The set of protein arginine methyltransferases (PRMTs) is a family of enzymes that catalyze the transfer of a methyl group from S-adenosyl-L-methionine (SAM) to the guanidino nitrogen of an arginyl residue to produce S-adenosyl-L-homo-cysteine (SAH) and methyl arginyl residues. TbPRMT6 is the homologue of HsPRMT6 in T. brucei with 31% amino acid identity. The overall monomeric structure of TbPRMT6 consists of three parts: a SAM-binding domain (residues 36–181, blue), a dimerization arm (residues 193–225, yellow), and a β-barrel domain (residues 182–192 and residues 230–368, green). The structures of TbPRMT6 highlight several structural features that are distinct from those found in previously characterized type I PRMTs, including four stretches of insertion, the absence of the β15 strand, and a unique dimerization arm.

Structures of apo-TbPRMT6 and in complex with SAH (SAH-TbPRMT6) were resolved and refined at 2.20 Å and 2.35 Å, respectively. The superimposition of the apo-TbPRMT6 structure with the SAH-TbPRMT6 structure revealed that the active site undergoes rearrangements upon SAH binding. Unlike the significant backbone motions observed in CARM1 and DOT1L active sites, cofactor binding primarily induced side-chain rearrangements in TbPRMT6 active site. Without SAH, the guanidine group of R39 of helix αZ and the imidazole ring of H318 of the THW loop point out from the active site. The comparison of the apo-TbPRMT6 and SAH-TbPRMT6 structures revealed the fine rearrangements of the TbPRMT6 active site upon SAH binding, which is critical for substrate binding, as demonstrated by an ITC assay.

>[4x]MESGGFAEDYDPNSSLHHQYYESYSDLAVHRLMLEDAQRMSFYRKSIEQSASIEGKVVVDVGSGTGILSMWAARAGAKHVFSIEASSLSEFQIGVVEDNDLSTKITVLGDTVENIIAGGVANFVNRHKAKLGKCGVAVLLSEWMGFYLFHEGMLPSVIRARNFFQDVNAALGVLQPIEMIPERATVFVAPITCKPYYVQRYKNFWRDVDGLDFSRYGRIEYEVYLEQASPLVECLPPLCLLHEGLSLIELNLSTVQEEVLTSLHNTVHFDLKESAEFQQHAREAGSEGRVSVDGFTVWFDVSYGAHTLSTSPRSPSTHWKQTTILLPREARNEELVSFPVEGGELGVEMHISASDKTLRFYTIELELK> MAHHHHHHAAMLRVAVPNKGALSEPATEILAEAGYRRRTDSKDLTVIDPVNNVEFFFLRPKDIAIYVGSGELDFGITGRDLVCDSGAQVRERLALGFGSSSFRYAAPAGRNWTTADLAGMRIATAYPNLVRKDLATKGIEATVIRLDGAVEISVQLGVADAIAD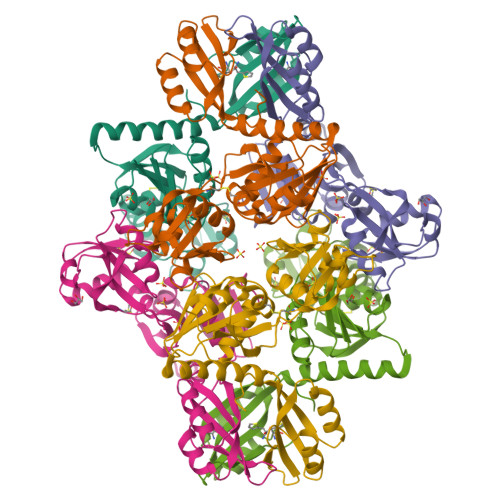VVGSGRTLSQHDLVAFGEPLCDSEAVLIERAGTDGQDQTEARDQLVARVQGVVFGQQYLMLDYDCPRSALKKATAITPGLESPTIAPLADPDWVAIRALVPRRDVNGIMDELAAIGAKAILASDIRFCRF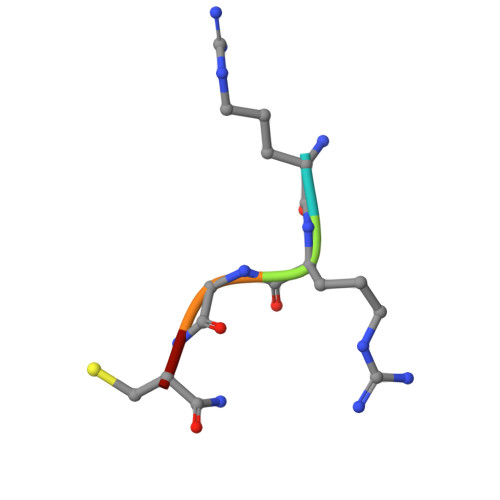> RRGCX> SKGENSKLNPWAVVGFIDAEGSFMVRVRKNSKYKTGWLVVAIFSVTVDKKDLFLLESLKTFFGGLGSIKKSGNSTFSYRIESSEQLTKIILPFFDKYSLITEALGDYLLFKKVLELMGTKEHLTQRGLEKIVSLKASINKGLSEELQAAFPQCVPTPRPEINNKNIPDPFWLAGFVSGDGSFKSILKKSESIKVGFQSILVFQITQHARDVKLMESLISYLGCGFIEKDSRGPWLYYTVTNFSDIQGKIIPFFHQYKIIGSAYGDYQDW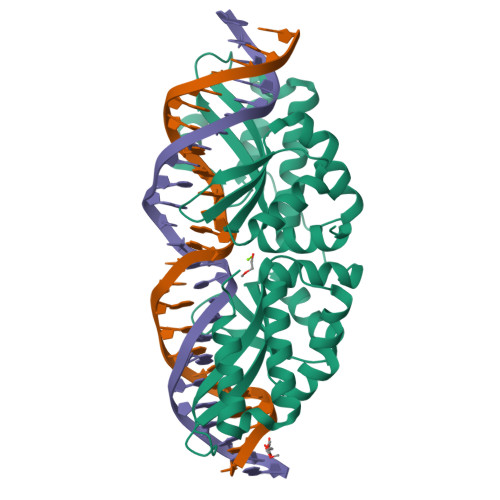CKIALIMQNKNHLTPEGLNEIRALKGGMNKGRL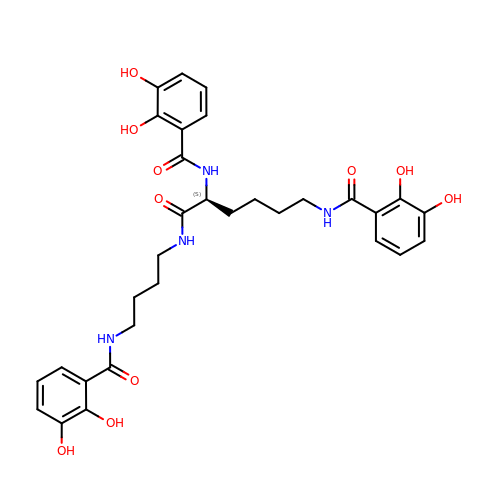~{N}-[(5~{S})-5-[[2,3-bis(oxidanyl)phenyl]carbonylamino]-6-[4-[[2,3-bis(oxidanyl)phenyl]carbonylamino]butylamino]-6-oxidanylidene-hexyl]-2,3-bis(oxidanyl)benzamide | C31 H36 N4 O10 | FRTUVWLJPRMTFC-NRFANRHFSA-N> MSRLEIYSPEGLRLDGRRWNELRRFESSINTHPHAADGSSYMEQGNNKIITLVKGPKEPRLKSQMDTSKALLNVSVNINKFSKFERSKSSHKNERRVLEIQTSLVRMFEKNVMLNIYPRTVIDIEIHVLEQDGGIMGSLINGITLALIDAGISMFDY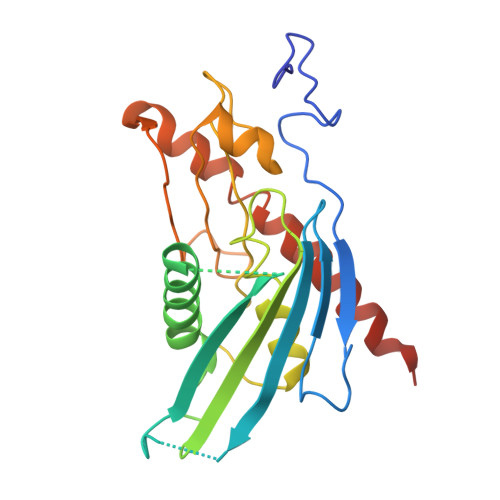ISGISVGLYDTTPLLDTNSLEENAMSTVTLGVVGKSEKLSLLLVEDKIPLDRLENVLAIGIAGAHRVRDLMDEELRKHAQKRVSNASAR>QMNYEEVIKKYKGNENFDHAAYDWRLHSGVTPVKDQKNCGSCWAFSSIGSVESQYAIRKNKLITLSEQELVDCSFKNYGCNGGLINNAFEDMIELGGICTDDDYPYVSDAPNLCNIDRCTEKYGIKNYL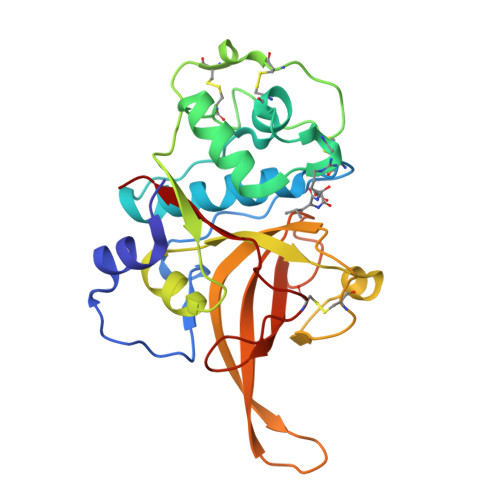SVPDNKLKEALRFLGPISISVAVSDDFAFYKEGIFDGECGDQLNHAVMLVGFGMKEIVNPLTKKGEKHYYYIIKNSWGQQWGERGFINIETDESGLMRKCGLGTDAFIPLIE[2x]> GNAKNKESPTKAIVRLRE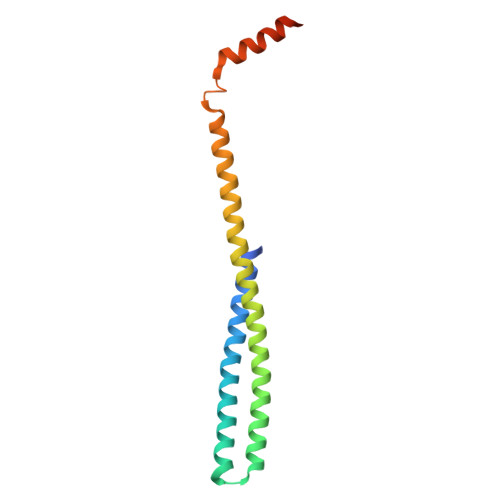HINLLSKKQSHLRTQITNQENEARIFLTKGNKVMAKNALKKKKTIEQLLSKVEGTMESMEQQLFSIESANLNLETMRAMQEGAKAMKTIHSGLDIDKVDETMDEIREQVELGDEISDAISRP> MNLHEYQAKEILARYGVPVPPGKVAYTPEEAKRIAEEFGKRVVIKAQVHVGGRGKAGGVKLADTPQEAYEKAQAILGMNIKGLTVKKVLVAEAVDIAKEYYAGLILDRAKKRVVLMLSKEGGVDIEEVAAERPEAIHKFWIDPHKGFRPFEAREMVKRAGLEGNLNKLAQVLVALYRAYEGVDASIAEINPLVVTTDGGIVAADAKIVLDDNALFRHPDLAELREVEAEHPLEVEASNYGFAYVKLDGNIGIIGNGAGLVMYTLDLVNRVGGKPANFLDIGGGAKADVVYNALKVVLKDPDVKGVFI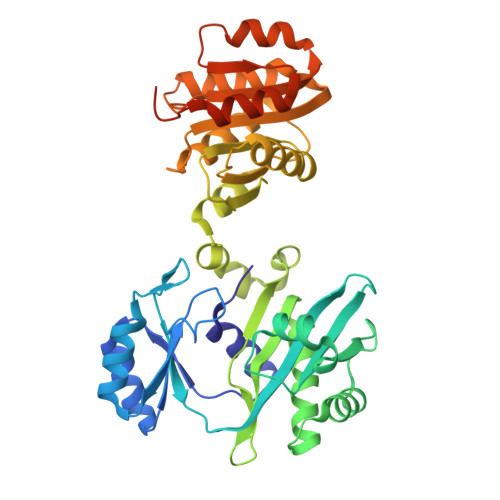NIFGGITRADEVAKGVIRALEEGLLTKPVVMRVAGTAEEEAKKLLEGKPVYMYPTSIEAAKVTVAMKGGAAWLEFAPGDLPMVHSQYNLL> ATYSTVPKIAFYAGLKRQHEGYEVLKFDDVVTNLGNHYDPTTGKFTCSIPGIYFFTYHVLMRGGDGTSMWADLCKNNQVRASAIAQDAAQNYDYASNSVVLHLEPGDEVYIKL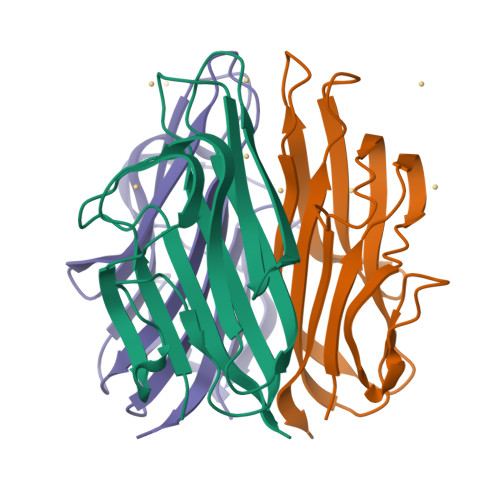DGGKAHGGNNNKYSTFSGFIIYAD> MHHHHHHQIGWRREGIKYRRNELFLDVLESVNLLMSPQGQVLSAHVSGRVVMKSYLSGMPECKFGMNDKIVIEKQGKGTADETSKSGKQSIAIDDCTFHQCVRLSKFDSERSISFIPPDGEFELMRYRTTKDIILPFRVIPLVREVGRTKLEVKVVIKSNFKPSLLAQKIEVRIPTPLNTSGVQVICMKGKAKYKASENAIVWKIKRMAGMKESQISAEIELLPTNDKKKWARPPISMNFEVPFAPSGLKVRYLKVFEPKLNYSDHDVIKWVRYIGRSGIYETRC;> SDLLAWDPLFG

Proper operation of the pivotal CME cargo adaptor AP2 requires membrane-localized Fer/Cip4 homology domain-only proteins (FCHO). The AP2 complex, composed of α, β2, μ2, and σ2 subunits, is pivotal to mammalian CCV formation, and its deletion is embryonically lethal in mice. FCHO1 and FCHO2 are similar in overall domain arrangement —folded N-terminal acidic phospholipid-binding homodimerization F-BAR domains and C-terminal folded μ-homology domains (μHD) separated by a ~300-residue, low-complexity intrinsically disordered protein linker, which has been suggested to participate in AP2 activation, although how it does so is undetermined. We dissect the network of interactions between the FCHO interdomain linker and AP2, which concentrates, orients, tethers, and partially destabilizes closed AP2 at the plasma membrane.

Crystals of a complex of Cμ2 and a peptide corresponding to this WxxL signal were grown, diffracted to 1.7-Å resolution, and were solved by MR using 1.9-Å unliganded Cμ2 as a search model. Binding was dependent on the presence of the tryptophan side chain as the homologous sequence from FCHO1, which does not contain a tryptophan, showed no binding. The mode favored will likely be context dependent, and it will likely be affected by multiple spatial and temporal factors in a nascent CCP including how many other α-appendage binding CCV proteins are present and whether the YxxΦ site of Cμ2 is accessible and/or occupied by cargo. These binding modes are likely to be in dynamic equilibrium with each other. The absence of WxxL in the C block of neuronally enriched FCHO1 but its presence in the ubiquitously expressed FCHO2 may reflect the paucity of YxxΦ-containing cargo found in synaptic CCVs that could compete out WxxL from Cμ2, which, if it did not occur, could slow or stall CCV formation. Thus, C blocks of all muniscin family members can bind to the α-appendage platform in a manner that is competitive with the binding of FxDxF and DP[FW] motifs of accessory CME proteins, and in addition, the partially overlapping WxxL sequence found only in FCHO2 can bind to the Cμ2 YxxΦ cargo–binding site and therefore potentially stabilize the unclosed but not-yet-open form of AP2.The second hitherto unknown bacterial proteasome family member was primarily found in Betaproteobacteria, hence its name BPH, short for Betaproteobacterial proteasome homologue. In this study, we present the first experimental characterization of two bacterial BPH proteins. Their crystal structures reveal homo-oligomeric double-barrel complexes with internalized active sites akin to those of proteasome and HslV. Unique structural features, however, like an elongated inner pore loop with a highly acidic sequence, distinguish BPH from its relatives. Confirming an initial hypothesis, our cluster analysis shows that BPH branches off from HslV and appears to be its direct descendant.

In crystallization trials, we obtained for Td-BPH a hexagonal crystal form diffracting to about 2.7 Å and an orthorhombic one diffracting to 2.3 Å. The higher-resolution orthorhombic crystal form could subsequently be solved in space group P212121 via molecular replacement, locating a single tetradecameric double ring in the ASU. The tetradecameric complexes from both crystal forms are virtually identical, and most of the sequence is resolved in all chains from Thr1 until Pro-190. However, in both crystal forms, the center portion of the pore loop (between Gln-95 and Glu-101) is disordered. In summary, both BPH proteins unequivocally form double rings with 7-fold symmetry in solution. Prominent residues in Td-BPH are Thr-1, Asp-17, and Lys-37, with Thr-1 acting as catalytic nucleophile. Lys-37 corresponds to Lys-33 in the proteasome; its function is to facilitate deprotonation of Thr-1 (28). Asp-17 assists in this reaction by orienting Lys-37 and making it prone to protonation. Equally present are e.g. conserved Gly-50, which helps to provide the oxyanion hole that stabilizes the transition state, and Ser-139, which forms hydrogen bonds with Thr-1. The S1 pocket, determining substrate specificity, is of hydrophobic character, priming it for the accommodation of uncharged amino acids.

>TTVTIVRKDGRIAIAADTLTKWGGGKESADYVANHEKIIRVGDSYVAITGSATFKLILADYFASLDEPPQLDSVARIFCVWNTLHGALKEHYYLQAGEDKEDDLESSRMDVLIANPRGIFGVAAHRTVQEFSKFYAYGSGSPYALGAMYAAYRAPSLDAEAVARLGVMAAAEFHDESGLPVQSFVMELSPDVGSGENLYFQ[14x]> GTGDGSELPKEMEEYFEMLQREIDKAYEIAKKARAQGKDPSLDVEIPQATDMAGRVESLVGPPGVAKRIRELVKEYGKEIAALKIVDEIIEGKFGDLGSREKYAEQAVRTALAILTEGIVSAPIEGIANVKIKRNTWADNSEYLALYYAGPIRSSGGTAQALSVLVGDYVRRKLGLDRFKPSEKHIERMVEEVDLYHRAVTRLQYHPSPEEVRLAMRNIPIEITGEATDDVEVSHRDVPGVETNQLRGGAILVLAEGVLQKAKKLVKYIDKMGIEGWEWLKEFVEAKEKGEPKEEGKEESLAESTLEETKVEVDMGFYYSLYQKFKEEIAPSDKYAKEVIGGRPLFSDPSKPGGFRLRYGRSRASGFATWGINPATMILVDEFLAIGTQLKTERPGKGAVVTPVTTIEGPIVKLKDGSVLRVDDYNLALKVREDVEEILYLGDAVIAFGDFVENNQTLLPANYCEEWWILEFVKALKEIYEVHLEPFTENEEESIEEASDYLEIDPEFLKEMLRDPLRVKPPVELAIHFSEVLGIPLHPYYTLYWNSVEPKDVEKLWRLLKNYAEIEWSNFRGIKFAKKIVISQEKLGDSKRTLELLGLPHTVRDGNVIVDYPWAAALLTPLGNLNWEFMAKPLYATIDIINENNEIKLRDRGISWIGARMGRPEKAKERKMKPPVQVLFPIGLAGGSSRDIKKAAEEGKVAEVEIAFFKCPKCGHVGPEHLCPNCGTRKELLWVCPRCNAEYPESQAEGYNYTCPKCNVKLRPYAKRKIRPSELLNRAMENVKVYGVDKLKGVMGMTSGWKMPEPLEKGLLRAKNDVYVFKDGTIRFDATDAPITHFRPREIGVSVEKLRELGYTHDFEGKPLVSEDQIVELKPQDIIL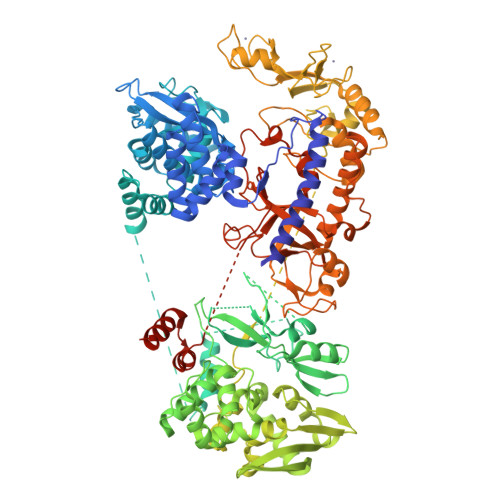SKEAGRYLLKVAKFVDDLLEKFYGLPRFYNAEKMEDLIGHLVIGLAPHTSAGIVGRIIGFVDALVGYAHPYFHAAKRRNCDGDEDAVMLLLDALLNFSRYYLPEKRGGKMDAPLVITTRLDPREVDSEVHNMDIVRYYPLEFYEATYELKSPKELVGVIERVEDRLGKPEMYYGLKFTHDTDDIAL> QYAPQTQSGRTSIVHLFEWRWVDIALECERYLGPKGFGGVQVSPPNENVVVTNPSRPWWERYQPVSYKLCTRSGNENEFRDMVTRCNNVGVRIYVDAVINHMCGSGAAAGTGTTCGSYCNPGSREFPAVPYSAWDFNDGKCKTASGGIESYNDPYQVRDCQLVGLLDLALEKDYVRSMIADYLNKLIDIGVAGFRIDASKHMWPGDIKAVLDKLHNLNTNWFPAGSRPFIFQEVIDLGGEAIKSSEYFGNGRVTEFKYGAKLGTVVRKWSGEKMSYLKNWGEGWGFMPSDRALVFVDNHDNQRGHGAGGSSILTFWDARLYKVAVGFMLAHPYGFTRVMSSYRWARNFVNGEDVNDWIGPPNNNGVIKEVTINADTTCGNDWVCEHRWREIRNMVWFRNVVDGEPFANWWDNGSNQVAFGRGNRGFIVFNNDDWQLSSTLQTGLPGGTYCDVISGDKVG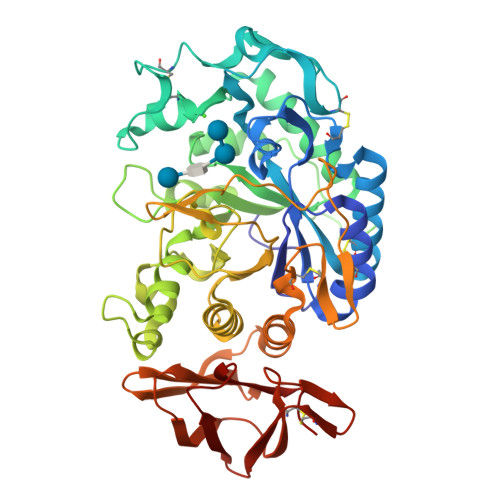NSCTGIKVYVSSDGTAQFSISNSAEDPFIAIHAESKL> MNECAFGTKDPVYLNYHDHVWGQPLYDSKALFKLLALESQHAGLSWLTILKKKEAYEEAFYDFEPEK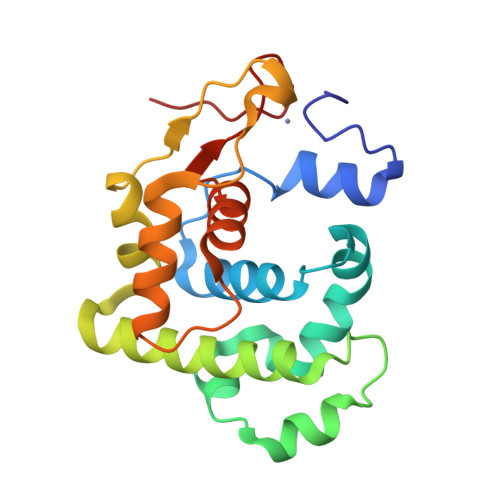VAQMTAQDIDRLMTFPNIVHHRKKLEAIVNQAQGYLKIEQAYGSFSKFLWSYVNGKPKDLQYEHASDRITVDDTATQLSKDLKQYGFKFLGPVTVFSFLEAAGLYDAHLKDCPSKPKHN>[2x]GSKPFSLPILTLSELTNSRFPVPIDSLFTAQNNVLQVQCQNGRCTLDGELQGTTQLLPTGICAFRGRVTAQINQRDRWHMQLQNLNGTTYDPTDDVPAPLGTPDFKGVVFGMVSQRNVGNDAPGSTRAQQAWVSTYSPQFVPKLGSVNLRISDNDDFQFQPTKFTPVGVNDDDDGHPFRQWELPNYSGELTLN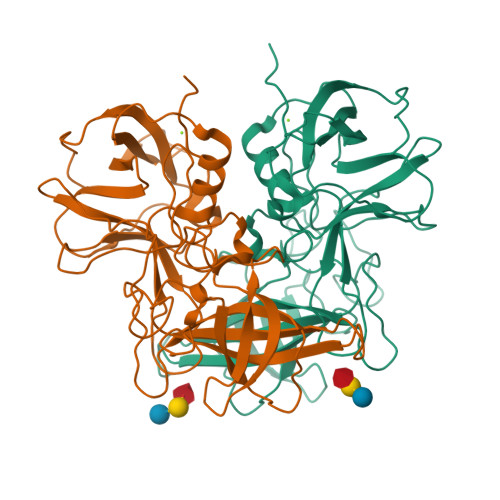MNLAPPVAPNFPGEQLLFFRSFVPCSGGYNQGIIDCLIPQEWIQHFYQESAPSQSDVALIRYVNPDTGRTLFEAKLHRSGYITVAHSGDYPLVVPANGHFRFDSWVNQFYSLAPM>[2x]MDRMKIEAVIFAWAGTTVDYGCFAPLEVFMEIFHKRGVAITAEEARKPMGLLKIDHVRALTEMPRIASEWNRVFRQLPTEADIQEMYEEFEEILFAILPRYASPINGVKEVIASLRERGIKI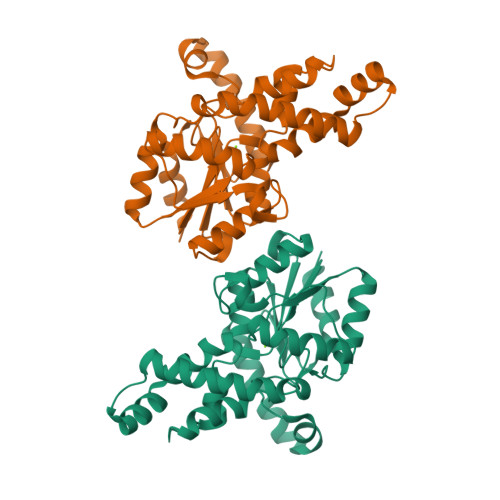GSTTGYTREMMDIVAKEAALQGYKPDFLVTPDDVPAGRPYPWMCYKNAMELGVYPMNHMIKVGDTVSDMKEGRNAGMWTVGVILGSSELGLTEEEVENMDSVELREKIEVVRNRFVENGAHFTIETMQELESVMEHIEKQELIIS> MRGSHHHHHHGSMPETNPNAPPRPDSLLNPSDALKHLEEYPRGDGLSLQELMDSRKNGGLTYNDFLVLPGHINFPASDVSLQSKATKNIVLNTPFLSSPMDTVTEDRMAIALALHGGLGIIHHNCSAEEQAAMVRRVKKYENGFITDPLCLGPDATVGDVLEIKAKFGFCGVPITETGEPDSKLLGIVTGRDVQFQDAETPIKSVMTTEVVTGSSPITLEKANSLLRETKKGKLPIVDSNGHLVSLVARSDLLKNQNYPYASKVPESKQLYCGAAIGTRPGDKDRLKLLAEAGLDVVVLDSSQGNSVYQIEFIKWIKQTYPKIDVIAGNVVTREQAAQLIAAGADGLRIGMGSGSICITQEVMAVGRPQGTAVYAVAEFASRFGIPCIADGGIGNIGHIAKALALGASAVMMGGLLAGTTESPGEYFYHEGKRVKVYRGMGSIEAMEHTQRGSASGKRSILGLDNAATARYFSEADAVKVAQGVSGDVADKGSINKFVPYLFTGLQHSLQDAAIKSVSELHSCARSGSLRFELRTASAQLEGGVHGLNSYTKRLFA;> MRGSHHHHHHGSMPETNPNAPPRPDSLLNPSDALKHLEEYPRGDGLSLQELMDSRKNGGLTYNDFLVLPGHINFPASDVSLQSKATKNIVLNTPFLSSPMDTVTEDRMAIALALHGGLGIIHHNCSAEEQAAMVRRVKKYENGFITDPLCLGPDATVGDVLEIKAKFGFCGVPITETGEPDSKLLGIVTGRDVQFQDAETPIKSVMTTEVVTGSSPITLEKANSLLRETKKGKLPIVDSNGHLVSLVARSDLLKNQNYPYASKVPESKQLYCGAAIGTRPGDKDRLKLLAEAGLDVVVLDSSQGNSVYQIEFIKWIKQTYPKIDVIAGNVVTREQAAQLIAAGADGLRIGMGSGSICITQEVMAVGRPQGTAVYAVAEFASRFGIPCIADGGIGNIGHIAKALALGASAVMMGGLLAGTTESPGEYFYHEGKRVKVYRGMGSIEAMEHTQRGSASGKRSILGLDNAATARYFSEADAVKVAQGVSGDVADKGSINKFVPYLFTGLQHSLQDAGIKSVSELHSCARSGSLRFELRTASAQLEGGVHGLNSYTKRLFA

IMPDH performs the rate-limiting, first step in de novo GTP biosynthesis, the NAD+-dependent conversion of inosine monophosphate (IMP) to xanthosine monophosphate (XMP) via a two-step oxidation and hydrolysis reaction. The catalytic mechanism of IMPDH involves a transition from a dehydrogenase to a hydrolase reaction; initially, the substrate IMP and cofactor NAD+ bind, IMP is then oxidized and forms a covalent transition state complex E-XMP* via a catalytic cysteine, while NAD+ is simultaneously reduced to NADH. The enzyme then undergoes a conformational change whereby a large mobile flap folds into the vacant NAD+ site, carrying a catalytic arginine residue that activates a water molecule to hydrolyze the E-XMP* covalent complex, releasing XMP. MPA is an NAD+ analogue and an uncompetitive inhibitor that traps the E-XMP* enzyme-substrate covalent complex by competing with the flap for the vacant NAD+ site.

To provide a foundation for fungus-specific inhibitor development, we determined the crystal structure of the clinically relevant C. neoformans var. grubii IMPDH in complex with the substrate IMP and the inhibitor MPA. CnImd1 forms a tetramer and in the final model each monomer contains 395 of the 544 residues in the typical eight-stranded α/β barrel structure, plus one molecule each of IMP and MPA bound in the active site, consistent with our functional observations suggesting an uncompetitive mechanism of enzyme inhibition. The large accessory subdomain between residues 130–244 and residues 438–449 from the mobile flap have no interpretable electron density, common to previous structural studies on this class of enzymes. MPA makes far fewer interactions in the cryptococcal IMPDH:IMP:MPA complex than observed in the hamster IMPDH structure, perhaps accounting for some of the differences in Ki between the mammalian and fungal enzyme. In particular, T347 (Cryptococcus numbering) faces away from the active site in the Cryptococcus enzyme and does not bind MPA, while several other residues including N317, D288 and G340 participate in fewer interactions with the ligands in the cryptococcal complex. Of note, one of the two residues responsible for MPA resistance in C. gattii VGIV IMPDH, R336 (K336 in the resistant enzyme), forms direct contacts with only IMP in the cryptococcal complex, suggesting a possible mechanistic explanation for the failure of the R336K single mutant to exhibit any altered sensitivity to MPA. The change in orientation of the loop in CnImd1 creates a large, Cryptococcus-specific pocket in the active site. The cryptococcal IMPDH structure is unique in having most of the mobile flap, except for 12 residues that encompass a small insertion region unique to Cryptococcus, sufficiently ordered to permit all but three residues corresponding to the flap in human IMPDH to be observed.> MSADSSPLVGSTPTGYGTLTIGTSIDPLSSSVSSVRLSGYCGSPWRVIGYHVVVWMMAGIPLLLFRWKPLWGVRLRLRPCNLAHAETLVIEIRDKEDSSWQLFTVQVQTEAIGEGSLEPSPQSQAEDGRSQAAVGAVPEGAWKDTAQLHKSEEAVSVGQKRVLRYYLFQGQRYIWIETQQAFYQVSLLDHGRSCDDVHRSRHGLSLQDQMVRKAIYGPNVISIPVKSYPQLLVDEALNPYYGFQAFSIALWLADHYYWYALCIFLISSISICLSLYKTRKQSQTLRDMVKLSMRVCVCRPGGEEEWVDSSELVPGDCLVLPQEGGLMPCDAALVAGECMVNESSLTGESIPVLKTALPEGLGPYCAETHRRHTLFCGTLILQARAYVGPHVLAVVTRTGFCTAKGGLVSSILHPRPINFKFYKHSMKFVAALSVLALLGTIYSIFILYRNRVPLNEIVIRALDLVTVVVPPALPAAMTVCTLYAQSRLRRQGIFCIHPLRINLGGKLQLVCFDKTGTLTEDGLDVMGVVPLKGQAFLPLVPEPRRLPVGPLLRALATCHALSRLQDTPVGDPMDLKMVESTGPQLQAMEEPPVPVSVLHRFPFSSALQRMSVVVAWPGATQPEAYVKGSPELVAGLCNPETVPTDFAQMLQSYTAAGYRVVALASKPLPTVPSLEAAQQLTRDTVEGDLSLLGLLVMRNLLKPQTTPVIQALRRTRIRAVMVTGDNLQTAVTVARGCGMVAPQEHLIIVHATHPERGQPASLEFLPMESPTAVNGVKDPDQAASYTVEPDPRSRHLALSGPTFGIIVKHFPKLLPKVLVQGTVFARMAPEQKTELVCELQKLQYCVGMCGDGANDCGALKAADVGISLSQAEASVVSPFTSSMASIECVPMVIREGRCSLDTSFSVFKYMALYSLTQFISVLILYTINTNLGDLQFLAIDLVITTTVAVLMSRTGPALVLGRVRPPGALLSVPVLSSLLLQMVLVTGVQLGGYFLTLAQPWFVPLNRTVAAPDNLPNYENTVVFSLSSFQYLILAAAVSKGAPFRRPLYTNVPFLVALALLSSVLVGLVLVPGLLQGPLALRNITDTGFKLLLLGLVTLNFVGAFMLESVLDQCLPACLRRLRPKRASKKRFKQLERELAEQPWPPLPAGPLR

ATP13A2 belongs to the orphan P5B adenosine triphosphatases (ATPase) family and has been established as a lysosomal polyamine exporter to maintain the normal function of lysosomes and mitochondria. Here, using single-particle cryo-EM, we present the structures of full-length human ATP13A2 in three distinct conformations including an E1 state (apo), an E1P-ADP state with ATP and Mg2+, and an E2-Pi state with SPM, phosphatidic acid (PA), and phosphatidylinositol(3,5)bisphosphate [PI(3,5)P2]. The structure of the human ATP13A2 adopts the typical P-type ATPase fold with overall dimensions of 125 Å × 75 Å × 70 Å, including ten transmembrane (TM) helices and three conserved cytoplasmic domains [N (nucleotide-binding) domain; A (actuator) domain; and P (phosphorylation) domain]. In addition, the P5B type ATP13A2 also comprises two specific domains: a C-terminal extension domain (CTD) laying close to the P-domain and an N-terminal domain (NTD) preceding the A domain showing amphipathic feature.

To investigate the possible SPM translocation mechanism of ATP13A2, we added SPM, PA, and PI(3,5)P2 during protein purification and sample preparation, and ultimately, we solve the structure of the E2-Pi state at a resolution of 3.6 Å. Comparison between this state and the E1P-ADP state reveals a door sliding motion formed by TM1 and TM2 accompanied by the rotation of the A domain and the tilt of the N domain. The conformational change in TMD creates a spindly negatively charged cavity that allows substrate entry from the lysosomal matrix. The SPM molecule is stabilized by extensive interactions between the amine nitrogen atoms groups from SPM and the acidic and aromatic side chains along the cavity. For instance, the amine nitrogen atoms are coordinated by D254, D463, D960, and D967 via hydrogen bonding interactions and by W251 and F963 via cation–π interactions. In addition, human ATP13A2 contains a narrow tunnel ― formed by TMs 1, 2, 4, 5, 6 ― than that of Spf1, due to the spindly character of the spermine substrate. The binding manner of the SPM substrate in these two structures is highly conserved. The E2P to E2-Pi transition is accompanied by the rearrangement of the A domain and the binding of SPM molecule in lysosomal lumen to the substrate cavity in the TMD of ATP13A2, thereby facilitating the dephosphorylation reaction. Interestingly, the E2P-inhibit state of Ypk9 reveals a long N terminal loop that interacts with the A- and N-domains and hijacks the ATPase in the E2P state. Such an auto-inhibition regulation mechanism is not observed in our current human ATP13A2 structures.>GSHMASMTGGQQMGRGSNNGDICIKDSINTLWTGINPPPNCQIVENTNTNDGKLTLVLVKNGGLVNGYVSLVGVSDTVNQMFTQKTANIQLRLYFDSSGNLLTEESDLKIPLKNKSSTATSETVASSKAFMPSTTAYPFNTTTRDSENYIHGICYYMTSYDRSLFPLNISIMLNS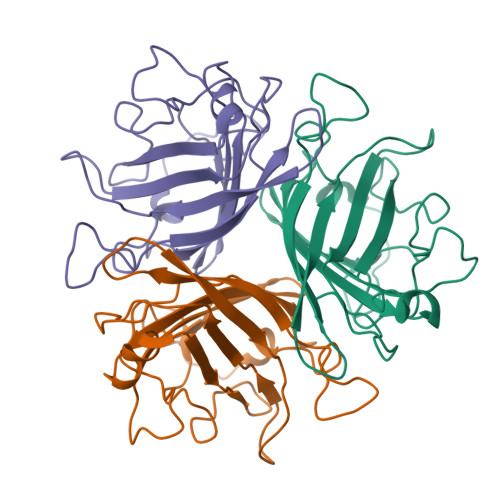RMISSNVAYAIQFEWNLNASESPESNIATLTTSPFFFSYITEDDN[6x]> MKQYLELMQKVLDEGTQKNDRTGTGTLSIFGHQMRFNLQDGFPLVTTKRCHLRSIIHELLWFLQGDTNIAYLHENNVTIWDEWADENGDLGPVYGKQWRAWPTPDGRHIDQITTVLNQLKNDPDSRRIIVSAWNVGELDKMALAPCHAFFQFYVADGKLSCQLYQRSCDVFLGLPFNIASYALLVHMMAQQCDLEVGDFVWTGGDTHLYSNHMDQTHLQLSREPRPLPKLIIKRKPESI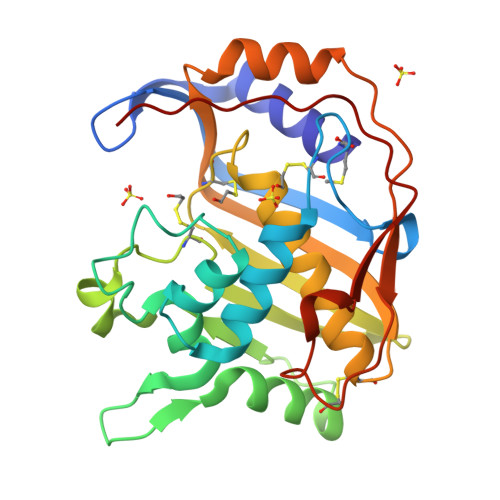FDYRFEDFEIEGYDSHPGIKAPVAI> GPHMLESRVSYDIEHLLYYSMSPHSWTLPTDWQKMQETAPSILRNKDLQDESQRFDGDKYLASIKTAA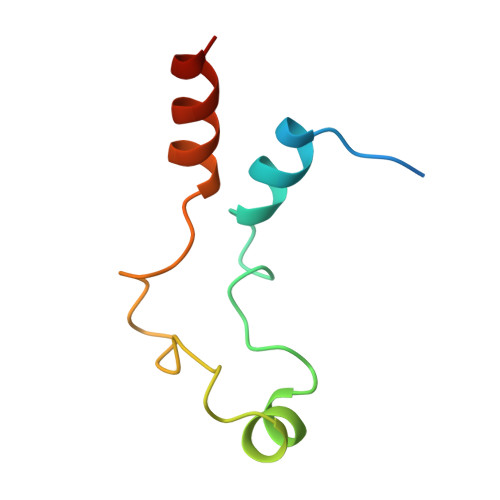KR>LSDSRVLWAPAEAHPLSPQGHPARLHRIVPRLRDVFGWGNLTCPICKGLFTAINLGLKKEPNVARVGSVAIKLCNLLKIAPPAVCQSIVHLFEDDMVEVWRRSVLSPSEACGLLLGSTCGHWDIFSSWNISLPTVPKPPPKPPSPPAPGAPVSRILFLTDLHWDHDYLEGTDPDCADPLCCRRGSGLPPASRPGAGYWGEYSKCDLPLRTLESLLSGLGPAGPFDMVYWTGDIPAHDVWHQTRQDQLRALTTVTALVRKFLGPVPVYPAVGNHESTPVNSFPPPFIEGNHSSRWLYEAMAKAWEPWLPAEALRTLRIGGFYALSPYPGLRLISLNMNFCSRENFWLLINSTDPAGQLQWLVGELQAAEDRGDKVHIIGHIPPGHCLKSWSWNYYRIVARYENTLAAQFFGHTHVDEFEVFYDEETLSRPLAVAFLAPSATTYIGLNPGYRVYQIDGNYSGSSHVVLDHETYILNLTQANIPGAIPHWQLLYRARETYGLPNTLPTAWHNLVYRMRGDMQLFQTFWFLYHKGHPPSEPCGTPCRLATLCAQLSARADSPALCRHLMPDGSLPEAQSLWPRPLFC[3x]

ASMD is a result of mutations in acid sphingomyelinase (ASM, E.C. 3.1.4.12), which hydrolyzes sphingomyelin to ceramide and phosphocholine. The structure includes an N-terminal saposin domain (residues 84–167), a proline-rich linker (168–195), a catalytic metallophosphatase domain (196–538), and a helical C-terminal domain (539–611). The substrate binding cleft in ASM is created by the catalytic domain in the middle, and saposin domain and C-terminal domain at two opposite sides. Zinc ions are prerequisites for activity of both forms.

Recombinant human ASM expressed from Chinese hamster ovary (CHO) cells is being developed as enzyme replacement therapy (ERT) for the non-neurological manifestations of ASMD, and is currently in the phase 1/2 pediatric trial and phase 2/3 trial for adults. The recombinant human ASM being developed for ERT, olipudase alfa, was also crystallized without any protease in the crystallization drops. Olipudase alfa was expressed in CHO cells with complex glycans. The olipudase alfa crystals diffracted to around 4 Å at synchrotron, and clear glycosylation and zinc cofactors densities were observed. Its refined structure was essentially identical to ASM from HEK cells. Clear electron density allowed us to build all residues from W84 to M611 as well as two zinc ions, six N-linked glycans, and eight disulfides. The same residue range is visible in the olipudase alfa structure, suggesting ASM N and C termini are inherently disordered and flexible.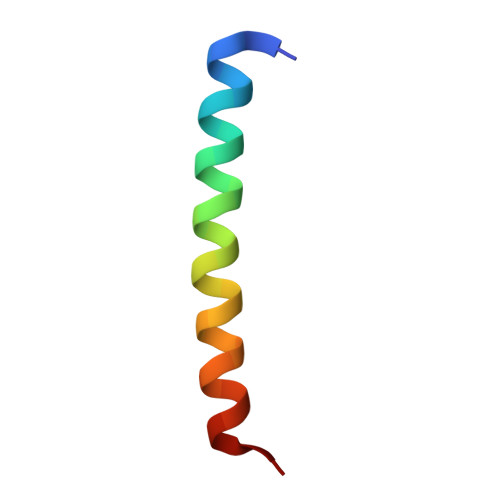> PDAYRFLTEQDRQLRLLQAQIQRLLEAQSLMP>GPLGSHMSTESNDGVSETLLAWRHIDFWTSEHNPDLNATLSDPCTQNDITHAEEDLEVSFPNPVKASFKIHDGQEDLESMTGTSGLFYGFQLMTLDQVVAMTQAWRNVAKNLNKRSQQGLSHVTSTGASSSMERLNGNKFKL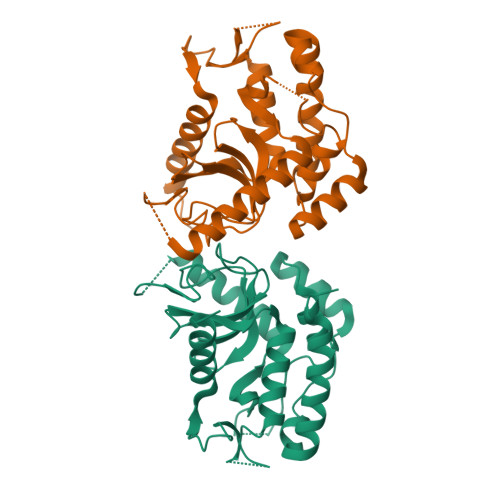PNIPDQKSIPPNAVQPVYAHPAWIPLITDNAGNHIGVDLAPGPNGKYAQIITFGRDFDTKFVIAENWGEFLLSFANDLEAGNWYLVDDNDDYFSGDGELVFRDKKSNGPIQDYFEVLKRRTWIKYQLERPHRD[2x]>MGSSHHHHHHSSGRENLYFQGMELLKHLSQRQYIDGEWVESANKNTRDIINPYNQEVIFTVSEGTKEDAERAILAARRAFESGEWSQETAETRGKKVRAIADKIKEHREALARLETLDTGKTLEESYADMDDIHNVFMYFAGLADKDGGEMIDSPIPDTESKIVKEPVGVVTQITPWNYPLLQASWKIAPALATGCSLVMKPSEITPLTTIRVFELMEEVGFPKGTINLILGAGSEVGDVMSGHKEVDLVSFTGSIETGKHIMKNAANNVTNIALELGGKNPNIIFDDADFELAVDQALNGGYFHAGQVCSAGSRILVQNSIKDKFEQALIDRVKKIKLGNGFDADTEMGPVISTEHRNKIESYMDVAKAEGATIAVGGKRPDRDDLKDGLFFEPTVITNCDTSMRIVQEEVFGPVVTVEGFETEQEAIQLANDSIYGLAGAVFSKDIGKAQRVANKLKLGTVWINDFHPYFAQAPWGGYKQSGIGRELGKEGLEEYLVSKHILTNTNPQLVNWFSK[4x]

We studied a putative BADH from an early MRSA COL isolate, denoted SaBADH, and showed that it is a functional NAD+-dependent BADH that utilizes BA as the primary substrate. BADHs are a group of enzymes from the aldehyde dehydrogenase (ALDH) superfamily that primarily catalyze the oxidation of betaine aldehyde (BA) to betaine; some BADHs also utilize other substrates. BADHs resemble ALDH in structure and are composed of a Rossmann-fold NAD(P)-binding domain, a catalytic (substrate-binding) domain and an oligomerization (bridging) domain. The solution data are supported by the structural analysis and emphasize the importance of the NAD+-driven structural rearrangements at the cofactor-binding and substrate-binding sites for enzymatic activity.

Among the previously functionally characterized SaBADH mutants, the Gly234Ser (G234S) mutant, G234S-SaBADH, had a higher affinity for NAD+ and decreased substrate inhibition, suggesting the existence of a structural and functional interaction between the NAD-binding and substrate-binding sites. Thus, this mutant was of particular interest and its structure determination in the apo and holo forms provides key atomic details on how the G234S substitution affects NAD+ binding. To fully understand the kinetic and inhibition mechanisms of G234S-SaBADH, we determined its crystal structures in apo and holo forms and in the presence/absence of BME and compared them with the wild-type structures. The first peptide stretch adopts a helical conformation extending helix αF in the presence of NAD+ and interacts with the adenine ring of the cofactor. Although this segment is unwound in apo SaBADHBME(+/−), it forms a similar helix turn in apo G234S-SaBADHBME(+/−) and apo SaBADHBME(+)PEG. NAD+ binding results in displacement of the Cα atoms of the second area by ∼1.6–1.9 Å. However, in apo G234S-SaBADHBME(−) and apo SaBADHBME(+)PEG Val288–Ser290 is also repositioned in an NAD-dependent manner. Firstly, the adenine ring of NAD+ imposes structural changes on helix αF that were also observed in apo G234S-SaBADHBME(+/−) and apo SaBADHBME(+)PEG. Difference electron-density peaks around the Ala212–Glu215 segment of the helix of these apo structures suggest that this region might be flexible in general and that NAD+ binding selects or induces the favorable conformational state.>MPTIDFTFCEINPKKGFGGANGNKISLFYNNELYMVKFPPKPSTHKEMSYT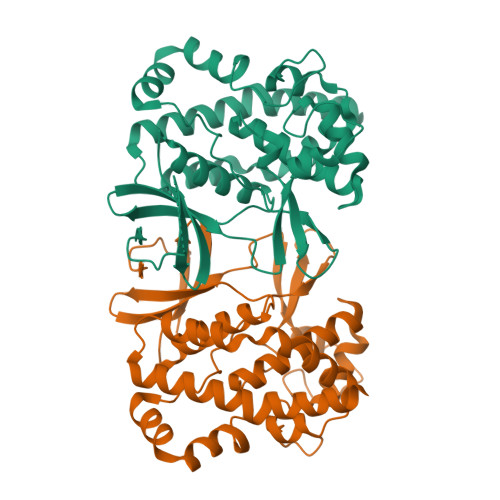NGCFSEYVACHIVNSLGLKVQETLLGTYKNKIVVACKDFTTHQYELVDFLSLKNTMIELEKSGKDTNLNDVLYAIDNQHFIEPKVLKCFFWDMFVADTLLGNFDRHNGNWGFLRASNSKEYQIAPIFDCGSCLYPQADDVVCQKVLSNIDELNARIYNFPQSILKDDNDKKINYYDFLTQTNNKDCLDALLRIYPRIDMNKIHSIIDNTPFMSEIHKEFLHTMLDERKSKIIDVAHTRAIELSLQHKQAHSNPYDNADDLDNSNEYTPTPKRRR[2x]>GSMSGVEQQVASLSGQCHHHGENLRELTTLLQKLQARVDQME[3x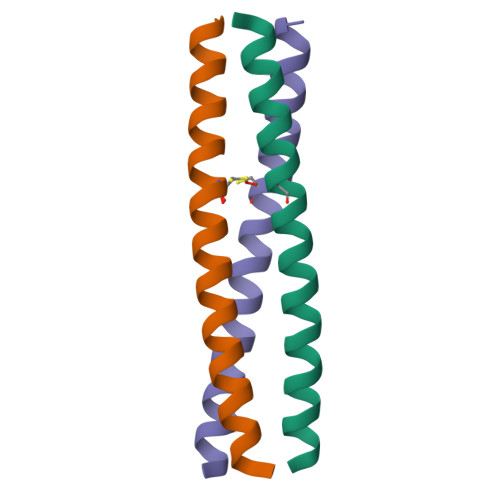]Toxin-antitoxin (TA) systems in prokaryotes are modules composed of a toxin and an antitoxin. All the MazF members are RNases, responsible for the cleavage of all types of RNAs participating in translation. Consequently, the activation of MazF RNases often leads to the inhibition of the translation process, reduction in metabolic rates, and eventually the formation of “persister cells”. Here, we report cocrystal structures of M. tb MazF-mt1 and -mt9, two important MazF members responsible for specific mRNA and tRNA cleavages, respectively, in complexes with truncated forms of their cognate antitoxin peptides.

In terms of the MazEF-mt1 TA system, our previous studies demonstrated that while η1 (Asp59-Arg76) did not bind to the cognate toxin, α3 (Thr42-Gly58) bound with a stronger affinity even greater than that of the full-length antitoxin. η1 was a small helix that follows α3, and the binding of η1 necessitates the conformational opening of the swapped loops (β1–β2) covering the MazF-mt1 dimer interface. Except for the two residues Trp54Ser55, the overall conformation and interactions are maintained in the cocrystal structure, when compared to that of the full-length MazE-mt1 complex. The close-up of the interaction details revealed that the peptide complex is maintained by the interactions on residues Tyr47 and Glu53-Ser55 of the α3-peptide. However, the last three residues of the peptide failed to maintain the helical shape with Trp54 of the antitoxin swinging to the other side. Additionally, the knot structure of MazF-mt1 became open due to the binding of the antitoxin peptide. Due to the extra energy needed to pry open this interface, the affinity of the MazF-mt1/MazE-mt1 complex is lower than the MazF-mt1/MazE-mt1 (α3). Interestingly, we found that the 4-nt RNA ACCU occupies the site that α3 binds. The α3-helix poses severe clashes against the 4-nt RNA fragment, which is a putative substrate/product. The tetranucleotide was probably from the cleaved substrate (the recognition site of MazF-mt1 is CU/ACC with “/” as the cleavage site), and the structure mimics the product-bound stage after the reaction. Although we failed to prove this point directly in our subsequent RNA-cleavage experiment due to unknown reasons, the strong affinity of α3 toward MazF-mt1 and the structural coincidence with the RNA fragment both suggested that the α3-helix would prevent the binding of the potential RNA substrate as well.

>GPELVMRRGEIWQVDLDPARGSEANNQRPAVVVSNDRANATATRLGRGVITVVPVTSNIAKVYPFQVLLSATTTGLQVDCKAQAEQIRSIATERLLRPIGRVSAAELAQLDEALKLHLDLWS[2x];> TLEDDYANAWQEWSAAG>SNAMMNQDIEKVLISEEQIQEKVLELGAIIAEDYKNTVPLAIGVLKGAMPFMADLLKRTDTYLEMDFMAVSSYGHSTVSTGEVKILKDLDTSVEGRDILIVEDIIDSGLTLSYLVDLFKYRKAKSVKIVTLLDKPTGRKVDLKADYVGFTVPHEFVVGYGLD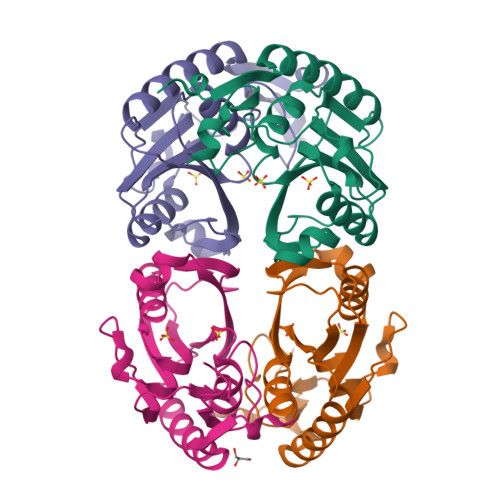YKEQYRNLPYVGVLKPSVYSN[4x]>GIKFSAEALRCHLRDHVNVSMVEVTDFPFNTSEWEGYLPKESIRTKAGPW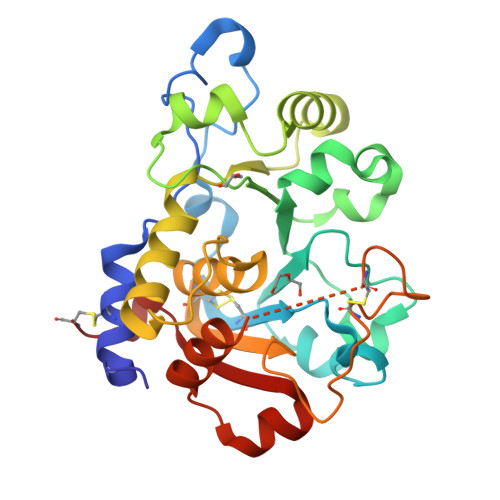GRCAVVSSAGSLKSSQLGREIDDHDAVLRFNGAPTANFQQDVGTKTTIRLMNSQLVTTEKRFLKDSLYNEGILIVWDPSVYHSDIPKWYQNPDYNFFNNYKTYRKLHPNQPFYILKPQMPWELWDILQEISPEEIQPNPPSSGMLGIIIMMTLCDQVDIYEFLPSKRKTDVCYYYQKFFDSACTMGAYHPLLYEKNLVKHLNQGTDEDIYLLGKATLPGFRTIHC[2x]Here, we characterize a two-component DRT9 system, composed of a reverse transcriptase (RT) and a non-coding RNA (ncRNA), which exhibits a protein-primed DNA synthesis activity upon phage infection. DRT9 system from Escherichia coli includes a 499 amino acids DRT9-RT protein and a 188 nucleotides ncRNA. DRT9-RT protein comprises five domains, including an N-terminal extension (NTE, residues 1–64) domain, a fingers domain (residues 65–159 and 176–211), a palm domain (residues 160–175 and 212–315), a thumb domain (residues 316–371 and 394–436) and a C-terminal extension (CTE, residues 372–393 and 437–499) domain. Structural analyses revealed that substrate-free DRT9 assembles as a dimer-of-dimers (tetrameric assembly), which undergoes an oligomeric reorganization into a trimer-of-dimers (hexameric assembly) upon substrate binding.

To elucidate the structural basis of DRT9-mediated immunity, we reconstituted and purified the DRT9-RT-ncRNA binary complex (hereafter referred to as DRT9) and determined its cryo-EM structure at a resolution of 3.49 Å. The overall structure of the DRT9 complex adopts a butterfly-like architecture assembled from four DRT9 protomers. Two DRT9 protomers, designated as A/A’ or B/B’, associate into an antiparallel, head-to-head dimer through the fingers, palm, and CTE domains of RT protein, constituting one wing of the butterfly-like structure. Two DRT9 dimers, referred to as wing-like units, further arrange in parallel to form a shoulder-to-shoulder tetramer through fingers and palm domains. A flipped uracil (U67) within SL4 inserts into a charged pocket formed by residues R205 and K208, generating essential cation-π and hydrogen-bonding interactions for dimer assembly. Specifically, the protruding SL5 of protomer B (or A’) from one wing engages a conserved loop region in protomer A (or B’) from the other wing, making C94-G114 Watson-Crick base pairs. In apo DRT9 tetramer, DRT_A/A’ and DRT_B/B’ dimer units are organized in parallel through interactions between the α10 helix and the assembly loop. In the DRT9 tetramer complex, the catalytic residues are fixed by two structural features, including a lysine-finger lock loop (residues 133–144) and a β-hairpin latch (residues 92-108). Specifically, two basic residues, K98 and R104 on the β-hairpin latch, form hydrogen bonds with D245. The R140 on the lock loop forms hydrogen bonds with D245 and D246.

>[4x]MKLEQQIQRVILEEAKALIKDYHEYHNRVHLESVRNKKRLGDSAPDKKIHRPNYWSFDKKFDPFYVKSNYKSIARSIANKIENRTYLPNEPFTKDVPKPDGGIRKVSIYQIPDAAISKLFFNRLLAKNRHRFSSFSYAYRNDRNVHFAIQDISVDLKKNERTFLAEFDFSDFFGSISHSFLNEQFNENGFYISPEEKFIIRSFLRERKVGIPQGTSISLFLANLTCWKLDQDLEREGVKFSRYADDTIIWSQEYSKICNAFNIITNFSKSAGIKINPKKSEGISLLTKKGLPSEITSKNNLDFLGYTLSVENVSIKEKSVKKIKKQISYILYRNLIQPLKKTSLAGQTIPANDRDKNFLIAICEIRRYMYGGLSKSQIKDYLSGRSNRLYFKGIMSFYPLVNDVEQLKQLDGWIVSVIYRALKLRCQLLSKWGYNRSHNFPFILDREDIVDKCSKKTIAGRKLFEIPSFLLIHKALQKGLQESGIEKIMNPQSLNYDYE>[2x]GAMDPEFGRPNPWDDKLIF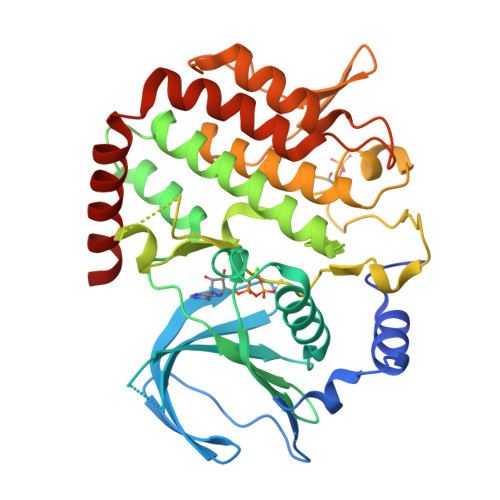KLLSGLSKPVSSYPNTFEWQCKLPAIKPKTEFQLGSKLVYVHHLLGEGAFAQVYEATQGDLNDAKNKQKFVLKVQKPANPWEFYIGTQLMERLKPSMQHMFMKFYSAHLFQNGSVLVGELYSYGTLLNAINLYKNTPEKVMPQGLVISFAMRMLYMIEQVHDCEIIHGDIKPDNFILGNGFLEQDDEDDLSAGLALIDLGQSIDMKLFPKGTIFTAKCETSGFQCVEMLSNKPWNYQIDYFGVAATVYCMLFGTYMKVKNEGGECKPEGLFRRLPHLDMWNEFFHVMLNIPDCHHLPSLDLLRQKLKKVFQQHYTNKIRALRNRLIVLLLECKRSRK>[2x]EHPEFLKAGKEPGLQIWRVEKFDLVPVPTNLYGDFFTGDAYVILKTVQLRNGNLQYDLHYWLGNECSQDESGAAAIFTVQL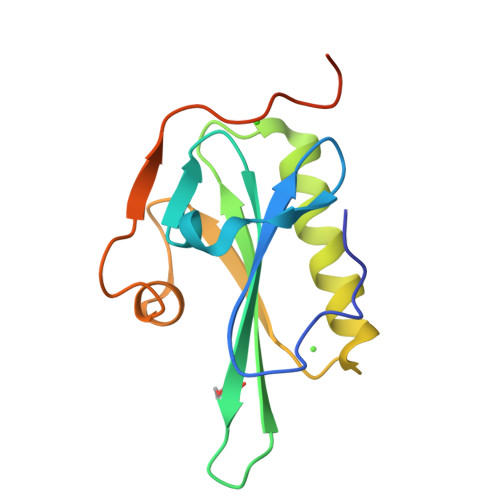DDYLNGRAVQHREVQGFESATFLGYFKSGLKYKKGGVASGFKHVVPNEVVVQR> XVNAKQYXRILK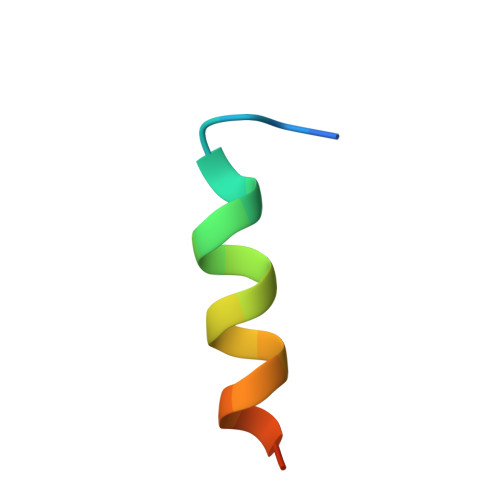RRXARAKLX> MNTRTIYLAGGSFWGLEAYFQRIDGVVDAVSGYANGNTKNPSYEDVSYRHTGHAETVKVTYDADKLSLDDILQYFFRVVDPTSLNKQGNDTGT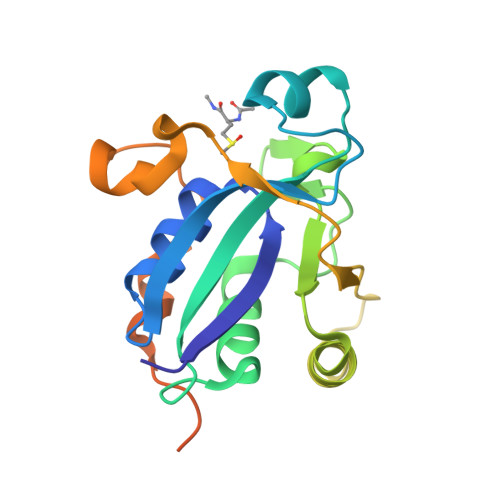QYRSGVYYTDPAEKAVIAAALKREQQKYQLPLVVENEPLKNFYDAEEYHQDYLIKNPNGYCHIDIRKADEPLPGKTKTAPQGKGFDAATYKKPSDAELKRT> MGHHHHHHMRKEIDPETSKYFSEIANLFDSNEVELEERSVICGNALEETRGREYEIATDYIISHVLQTLLEGCELDQLCSFIRNSASVFPAIAMDRSGSHVAESALKSLATHLENPDAYSVIEEALHSICKVIVDNPLDMMCNCYGSHVLRRLLCLCKGVPHQGFPGMLTYLLSGLLSCSREDMKYLQVDQYSSLVLQTALRLMLKQDEQL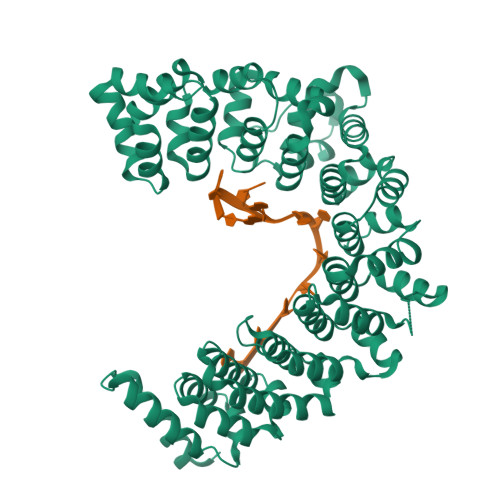LEIIPLILRCNSTNKKVEGFHIETNVAKEILESMKDNSFSHLVEVILEVAPESLYNEMFNKVFKNSLFELSVDRCANFVIQALISHARDQEQMGIMWEELAPRFKDLLEQGKSGVVASLIAVSQRLQSHENKCCEALVGAVCSTNESRISILPRLLFLDYYFGCRDKSTWEWAPGAKMHVMGCLILQGIFKFSSDHIQPYITSLTSMKAEYITETAKDSSGARVIEAFLASDAATKQKRRLIIKLRGHFGELSLHTSGSFTVEKCFDACNLTLREAIASELLDVKVDLSKTKQGPYLLRKLDIDGYASRPDQWKSRQEAKQSTYNEFCSAFGSNK> AE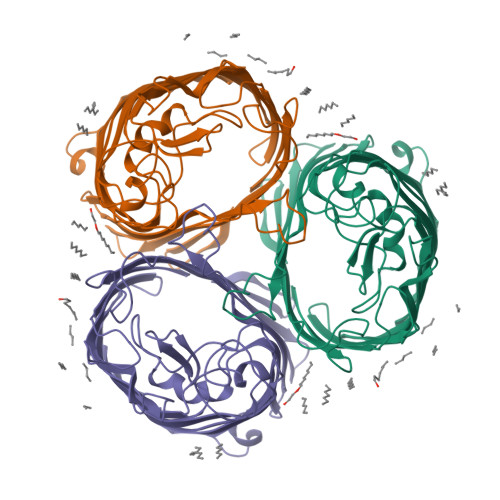IYNKDGNKVDLYGKAVGLHYFSKGNGENSYGGNGDMTYACLGFKGETQINSDLTGYGQWEYNFQGNNSEGADAQTGNKTRLAFAGLKYADVGSFDYGRNYGVVYDALGYTDMLPEFGGDTAYSDDFFVGRVGGVATYRNSNFFGLVDGLNFAVQYLGKNERDTARRSNGDGVGGSISYEYEGFGIVGAYGAADRTNLQEAQPLGNGKKAEQWATGLKYDANNIYLAANYGETRNATPITNKFTNTSGFANKTQDVLLVAQYQFDFGLRPSIAYTKSKAKDVEGIGDVDLVNYFEVGATYYFNKNMSTYVDYIINQIDSDNKLGVGSDDTVAVGIVYQF> KPFANTKKTLENQVEELTEKCSLKTDEFLKAKEKINEIFEKLNTI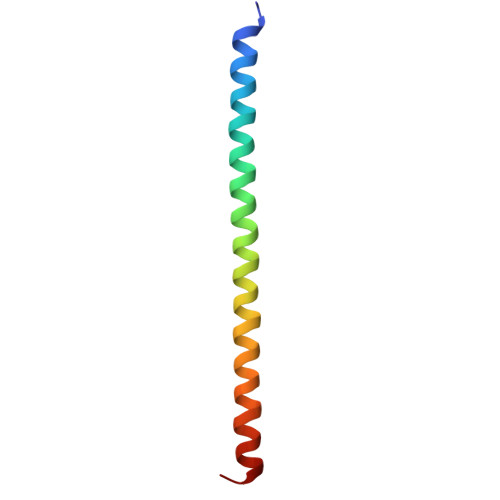RDEVIKKKNQNEYYR>NPMEAMYPHIFYFHFKNLRKAYGRNESWLCFTM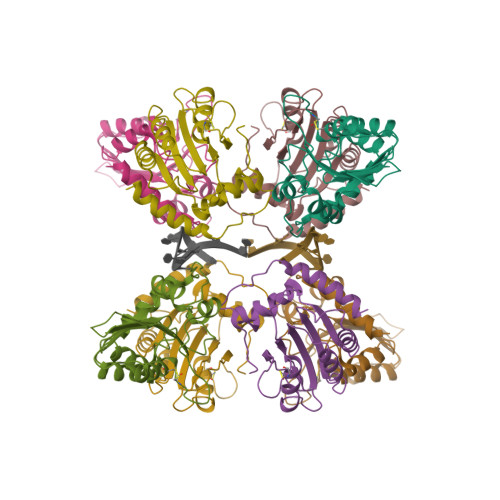EVVKHHSPVSWKRGVFRNQVDPETHCHAERCFLSWFCDDILSPNTNYEVTWYTSWSPCPECAGEVAEFLARHSNVNLTIFTARLYYFWDTDYQEGLRSLSQEGASVEIMGYKDFKYCWENFVYNDDEPFKPWKGLKYNFLFLDSKLQEILE[8x]> TPRSARLERMAQALALQAG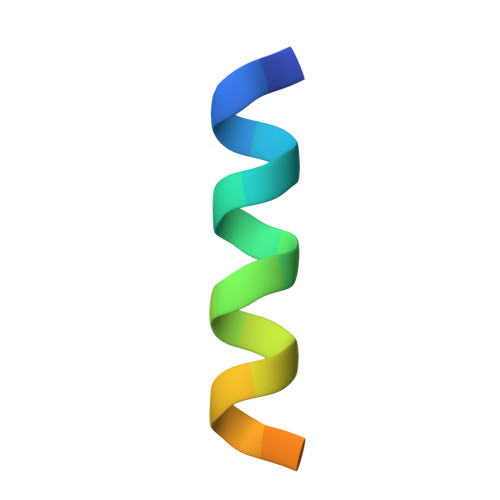SP>AAAAAAMTMMDMNFKYCHKIMKKHSKSFSYAFDLLPEDQRKAVWA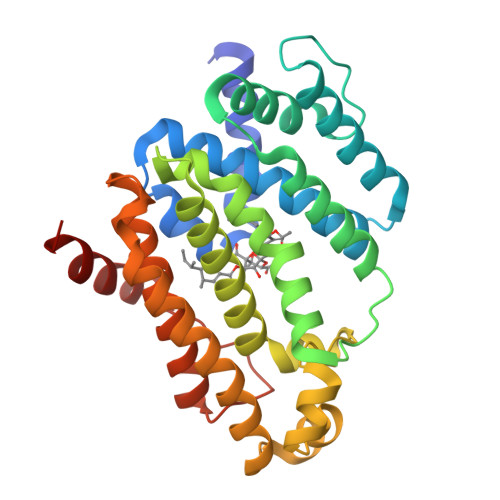IYAVCRKIDDSIDVYGDIQFLNQIKEDIQSIEKYPYEYHHFQSDRRIMMALQHVAQHKNIAFQSFYNLIDTVYKDQHFTMFETDAELFGYCYGVAGTVGEVLTPILSDHETHQTYDVARRLGESLQLINILRDVGEDFENERIYFSKQRLKQYEVDIAEVYQNGVNNHYIDLWEYYAAIAEKDFRDVMDQIKVFSIEAQPIIELAARIAIEILDEVRQANYTLHERVFVEKRKKAKLFHEINSKYHRI[2x]>[2x]AGKA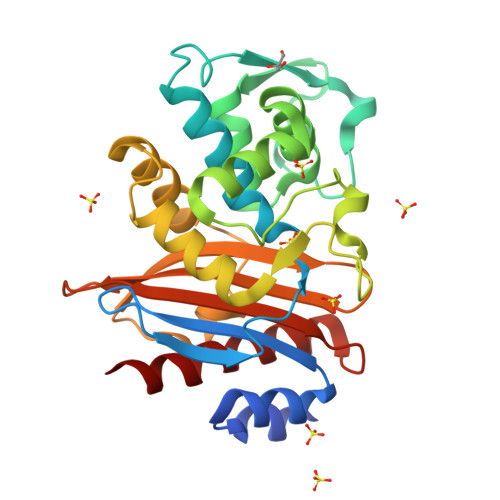TANAPTDAAITAASDFAALEKACAGRLGVTLLDTASGRRIGHRQDERFPMCSTFKSMLAATVLSQAERMPALLDRRVPVGEADLLSHAPVTRRHAGKDMTVRDLCRATIITSDNTAANLLFGVVGGPPAVTAFLRASGDTVSRSDRLEPELNSFAKGDPRDTTTPAAMAATLQRVVLGEVLQPASRQQLADWLIDNETGDACLRAGLGKRWRVGDKTGSNGEDARNDIAVLWPVAGGAPWVLTAYLQAGAISYEQRASVLAQVGRIADRLIG> MMETERLVLPPPDPLDLPLRAVELGCTGHWELLNLPGAPESSLPHGLPPCAPDLQQEAEQLFLSSPAWLPLHGVEHSARKWQRKTDPWSLLAVLGAPVPSDLQAQRHPTTGQILGYKEVLLENTNLSATTSLSLRRPPGPASQSLWGNPTQYPFWPGGMDEPTITDLNTREEAEEEIDFEKDLLTIPPGFKKGMDFAPKDCPTPAPGLLSLSCMLEPLDLGGGDEDENEAVGQPGGPRGDTVSASPCSAPLARASSLEDLVLKEASTAVSTPEAPEPPSQEQWAIPVDATSPVGDFYRLIPQPAFQWAFEPDVFQKQAILHLERHDSVFVAAHTSAGKTVVAEYAIALAQKHMTRTIYTSPIKALSNQKFRDFRNTFGDVGLLTGDVQLHPEASCLIMTTEILRSMLYSGSDVIRDLEWVIFDEVHYINDVERGVVWEEVLIMLPDHVSIILLSATVPNALEFADWIGRLKRRQIYVISTVTRPVPLEHYLFTGNSSKTQGELFLLLDSRGAFHTKGYYAAVEAKKERMSKHAQTFGAKQPTHQGGPAQDRGVYLSLLASLRTRAQLPVVVFTFSRGRCDEQASGLTSLDLTTSSEKSEIHLFLQRCLARLRGSDRQLPQVLHMSELLNRGLGVHHSGILPILKEIVEMLFSRGLVKVLFATETFAMGVNMPARTVVFDSMRKHDGSTFRDLLPGEYVQMAGRAGRRGLDPTGTVILLCKGRVPEMADLHRMMMGKPSQLQSQFRLTYTMILNLLRVDALRVEDMMKRSFSEFPSRKDSKAHEQALAELTKRLGALEEPDMTGQLVDLPEYYSWGEELTETQHMIQRRIMESVNGLKSLSAGRVVVVKNQEHHNALGVILQVSSNSTSRVFTTLVLCDKPLSQDPQDRGPATAEVPYPDDLVGFKLFLPEGPCDHTVVKLQPGDMAAITTKVLRVNGEKILEDFSKRQQPKFKKDPPLAAVTTAVQELLRLAQAHPAGPPTLDPVNDLQLKDMSVVEGGLRARKLEELIQGAQCVHSPRFPAQYLKLRERMQIQKEMERLRFLLSDQSLLLLPEYHQRVEVLRTLGYVDEAGTVKLAGRVACAMSSHELLLTELMFDNALSTLRPEEIAALLSGLVCQSPGDAGDQLPNTLKQGIERVRAVAKRIGEVQVACGLNQTVEEFVGELNFGLVEVVYEWARGMPFSELAGLSGTPEGLVVRCIQRLAEMCRSLRGAARLVGEPVLGAKMETAATLLRRDIVFAASLYTQ;> GPDSSQCESPSLTELFQEHKENNISQCFTLSDLCNQSSASFTDLSLGSFPLSQLANRCQSSPGISELTGSLSSLAFHKASPTRDLENLSLSELIAETIDVDNSQIKKESFEVSLSEVRSPGIDSNIDLSVLIKNPDFVPKPVVDPSIAPSSRTKVLSSKLGKNSNFAKDNKKNNKGSLTRKPPFSLSWTKALAARPSAFASTLCLRYPLKSCKRRTLDLYKTFLYSRQVQDVKDKEISPLVAITPFDFKSASPDDIVKANQKKAFTRELEVLFQ;> GPDSMASVTLSEAEKVYIVHGVQEDLRVDGRGCEDYRCVEVETDVVSNTSGSARVKLGHTDILVGVKAEMGTPKLEKPNEGYLEFFVDCSASATPEFEGRGGDDLGTEIANTLYRIFNNKSSVDLKTLCISPREHCWVLYVDVLLLECGGNLFDAISIAVKAALFNTRIPRVRVLEDEEGSKDIELSDDPYDCIRLSVENVPCIVTLCKIGYRHVVDATLQEEACSLASLLVSVTSKGVVTCMRKVGKGSLDPESIFEMMETGKRVGKVLHASLQSVVHKEESLGPKRQKVGFLG;> MPGDHRRIRGPEESQPPQLYAADEEEAPGTRDPTRLRPVYARAGLLSQAKGSAYLEAGGTKVLCAVSGPRQAEGGERGGGPAGAGGEAPAALRGRLLCDFRRAPFAGRRRRAPPGGCEERELALALQEALEPAVRLGRYPRAQLEVSALLLEDGGSALAAALTAAALALADAGVEMYDLVVGCGLSLAPGPAPTWLLDPTRLEEERAAAGLTVALMPVLNQVAGLLGSGEGGLTESWAEAVRLGLEGCQRLYPVLQQSLVRAARRRGAAAQP;> GPDSMAEPASVAAESLAGSRARAARTVLGQVVLPGEELLLPEQEDAEGPGGAVERPLSLNARACSRVRVVCGPGLRRCGDRLLVTKCGRLRHKEPGSGSGGGVYWVDSQQKRYVPVKGDHVIGIVTAKSGDIFKVDVGGSEPASLSYLSFEGATKRNRPNVQVGDLIYGQFVVANKDMEPEMVCIDSCGRANGMGVIGQDGLLFKVTLGLIRKLLAPDCEIIQEVGKLHPLEIVFGMNGRIWVKAKTIQQTLILANILEACEHMTSDQRKQIFSRLAES;> GPDSMAMEMRLPVARKPLSERLGRDTKKHLVVPGDTITTDTGFMRGHGTYMGEEKLIASVAGSVERVNKLICVKALKTRYIGEVGDIVVGRITEVQQKRWKVETNSRLDSVLLLSSMNLPGGELRRRSAEDELAMRGFLQEGDLISAEVQAVFSDGAVSLHTRSLKYGKLGQGVLVQVSPSLVKRQKTHFHDLPCGASVILGNNGFIWIYPTPEHKEEEAGGFIANLEPVSLADREVISRLRNCIISLVTQRMMLYDTSILYCYEASLPHQIKDILKPEIMEEIVMETRQRLLEQEG;> GPDSMAPPVRYCIPGERLCNLEEGSPGSGTYTRHGYIFSSLAGCLMKSSENGALPVVSVVRETESQLLPDVGAIVTCKVSSINSRFAKVHILYVGSMPLKNSFRGTIRKEDVRATEKDKVEIYKSFRPGDIVLAKVISLGDAQSNYLLTTAENELGVVVAHSESGIQMVPISWCEMQCPKTHTKEFRKVARVQPEFLQT;> GPDSMKETPLSNCERRFLLRAIEEKKRLDGRQTYDYRNIRISFGTDYGCCIVELGKTRVLGQVSCELVSPKLNRATEGILFFNLELSQMAAPAFEPGRQSDLLVKLNRLMERCLRNSKCIDTESLCVVAGEKVWQIRVDLHLLNHDGNIIDAASIAAIVALCHFRRPDVSVQGDEVTLYTPEERDPVPLSIHHMPICVSFAFFQQGTYLLVDPNEREERVMDGLLVIAMNKHREICTIQSSGGIMLLKDQVLRCSKIAGVKVAEITELILKALENDQKVRKEGGKFGFAESIANQRITAFKMEKAPIDTSDVEEKAEEIIAEAEPPSEVVSTPVLWTPGTAQIGEGVENSWGDLEDSEKEDDEGGGDQAIILDGIKMDTGVEVSDIGSQDAPIILSDSEEEEMIILEPDKNPKKIRTQTTSAKQEKAPSKKPVKRRKKKRAAN;> MAGLELLSDQGYRVDGRRAGELRKIQARMGVFAQADGSAYIEQGNTKALAVVYGPHEIRGSRARALPDRALVNCQYSSATFSTGERKRRPHGDRKSCEMGLQLRQTFEAAILTQLHPRSQIDIYVQVLQADGGTYAACVNAATLAVLDAGIPMRDFVCACSAGFVDGTALADLSHVEEAAGGPQLALALLPASGQIALLEMDARLHEDHLERVLEAAAQAARDVHTLLDRVVRQHVREASILLGD;> GPMLQKREKVLLLRTFQGRTLRIVREHYLRPCVPCHSPLCPQPAACSHDGKLLSSDVTHYVIPDWKVVQDYLEILEFPELKGIIFMQTACQAVQHQRGRRQYNKLRNLLKDARHDCILFANEFQQCCYLPRERGESMEKWQTRSIYNAAVWYYHHCQDRMPIVMVTEDEEAIQQYGSETEGVFVITFKNYLDNFWPDLKAAHELCDSILQSRRERENESQESHGKEYPEHLPLEVLEAGIKSGRYIQGILNVNKHRAQIEAFVRLQGASSKDSDLVSDILIHGMKARNRSIHGDVVVVELLPKNEWKGRTVALCENDCDDKASGESPSEPMPTGRVVGILQKNWRDYVVTFPSKEEVQSQGKNAQKILVTPWDYRIPKIRISTQQAETLQDFRVVVRIDSWESTSVYPNGHFVRVLGRIGDLEGEIATILVENSISVIPFSEAQMCEMPVNTPESPWKVSPEEEQKRKDLRKSHLVFSIDPKGCEDVNDTLSVRTLNNGNLELGVHIADVTHFVAPNSYIDIEARTRATTYYLADRRYDMLPSVLSADLCSLLGGVDRYAVSIMWELDKASYEIKKVWYGRTIIRSAYKLFYEAAQELLDGNLSVVDDIPEFKDLDEKSRQAKLEELVWAIGKLTDIARHVRAKRDGCGALELEGVEVCVQLDDKKNIHDLIPKQPLEVHETVAECMILANHWVAKKIWESFPHQALLRQHPPPHQEFFSELRECAKAKGFFIDTRSNKTLADSLDNANDPHDPIVNRLLRSMATQAMSNALYFSTGSCAEEEFHHYGLALDKYTHFTSPIRRYSDIVVHRLLMAAISKDKKMEIKGNLFSNKDLEELCRHINNRNQAAQHSQKQSTELFQCMYFKDKDPATEERCISDGVIYSIRTNGVLLFIPRFGIKGAAYLKNKDGLVISCGPDSCSEWKPGSLQRFQNKITSTTTDGESVTFHLFDHVTVRISIQASRCHSDTIRLEIISNKPYKIPNTELIHQSSPLLKSELVKEVTKSVEEAQLAQEVKVNIIQEEYQEYRQTKGRSLYTLLEEIRDLALLDVSNNYGI;> GPDSMAAGFKTVEPLEYYRRFLKENCRPDGRELGEFRTTTVNIGSISTADGSALVKLGNTTVICGVKAEFAAPSTDAPDKGYVVPNVDLPPLCSSRFRSGPPGEEAQVASQFIADVIENSQIIQKEDLCISPGKLVWVLYCDLICLDYDGNILDACTFALLAALKNVQLPEVTINEETALAEVNLKKKSYLNIRTHPVATSFAVFDDTLLIVDPTGEEEHLATGTLTIVMDEEGKLCCLHKPGGSGLTGAKLQDCMSRAVTRHKEVKKLMDEVIKSMKPK;> GPDSMEEETHTDAKIRAENGTGSSPRGPGCSLRHFACEQNLLSRPDGSASFLQGDTSVLAGVYGPAEVKVSKEIFNKATLEVILRPKIGLPGVAEKSRERLIRNTCEAVVLGTLHPRTSITVVLQVVSDAGSLLACCLNAACMALVDAGVPMRALFCGVACALDSDGTLVLDPTSKQEKEARAVLTFALDSVERKLLMSSTKGLYSDTELQQCLAAAQAASQHVFRFYRESLQRRYSKS

The ribonuclease in these processes is the RNA exosome complex, which degrades transcripts in a 3′–5′ direction and in a processive manner. The helicase can extract mRNA from the ribosome and is expected to transfer it to the exoribonuclease core through a bridging factor, HBS1L3 (also known as SKI7), but the mechanisms of this molecular handover remain unclear. We show that rather than a sequential handover, a direct physical coupling mechanism takes place, which culminates in the formation of a cytoplasmic exosome–ribosome supercomplex. Exosome and ribosome thus work together as a single structural and functional unit in co-translational mRNA decay, coordinating their activities in a transient supercomplex.

For structural characterization, we incubated the 80S-bound CrPV-IRES RNA with ATP and with EXO10-SKI containing an active SKI2 and an inactive DIS3L (D486N mutant), with the rationale of extracting the RNA substrate from the 80S but preventing degradation when the substrate 3′ end would reach the exosome exoribonuclease site. Signal subtraction of the 80S combined with focused three-dimensional (3D) classification, subsequent refinement and post-processing resulted in a reconstruction with nominal resolution ranging from 3.3 Å at the core to 8.7 Å in the outer regions. Human EXO9 has the typical barrel-like structure, with a lower ring of six RNase PH-like proteins (RRP41, RRP42, RRP43, RRP45, RRP46 and MTR3) and an upper ring of three S1–KH (‘cap’) proteins (RRP4, RRP40 and CSL4)10,11. A notable difference from nuclear EXO9-containing complexes is that a long segment of the RRP45CTD (residues 281–351) becomes structured as it wraps around roughly half of the EXO9 outer circumference. The DIS3L subunit contains an endonuclease-like PIN domain and an RNase II-like exoribonuclease domain that interact with the lower ring of EXO9. Second, DIS3L contains a C-terminal domain that binds to EXO9 by inserting between the RNase PH domain and the RRP45CTD. The outer surface of EXO10 presented additional densities, which we could attribute to three separate patches of SKI7EXO. In the first patch, SKI7 binds with a short helix (amino acids 555–572) in a cleft at the RRP43–MTR3 interface, consistent with mutagenesis data, and is further encased by the RRP45CTD. The third binding patch is located at the EXO9 upper ring, where SKI7 (residues 602–616) binds at the cap protein CSL4. From here, SKI7 residues 617–632 protrude into solvent with a highly conserved α-helix that extends towards the SKI2 catalytic core, engaging it in direct interactions at the RecA1 domain.> MAGNMLANYVQVYVMLPLDVVSVDNKFEKGDEIRAQLKKLTEAGVDGVMIDVWWGLVEGKGPKAYDWSAYKQVFDLVHEAGLKLQAIMSFHQCGGNVGDVVNIPIPQWVRDVGATDPDIFYTNRGGTRNIEYLTLGVDDQPLFHGRTAVQMYADYMASFRENMKKFLDAGTIVDIEVGLGPAGEMRYPSYPQSQGWVFPGIGEFICYDKYLEADFKAAAAKAGHPEWELPDDAGEYNDTPEKTQFFKDNGTYLTEKGKFFLSWYSNKLIKHGDKILDEANKVFLGCRVQLAIKISGIHWWYRVPNHAAELTAGYYNLDDRDGYRTIARMLTRHHASMNFTCAEMRDSEQSEEAKSAPEELVQQVLSAGWREGLHVACENALGRYDATAYNTILRNARPKGINKNGPPEHKLFGFTYLRLSNELLEGQNYATFQTFVEKMHANL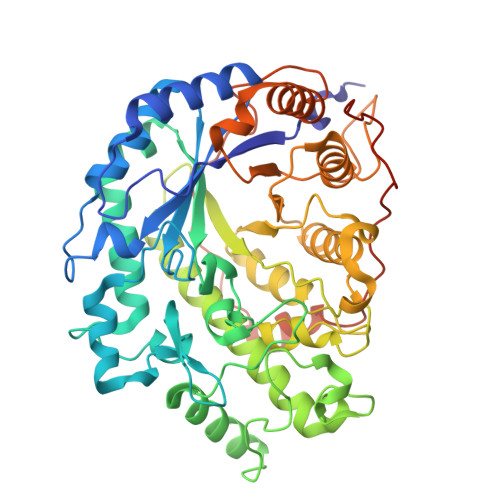GHDPSVDPVAPLERSKPEMPIEMILKAAQPKLEPFPFDKNTDLPVKDHTDVGDEVLVAPVHHHHHH>[4x]MVTALNYRVIDVDNHYYEPLDSFTRHLDKKFKRRGVQMLSDGKRTWAVIGDRVNHFIPNPTFDPIIVPGCLDLLFRGEIPDGVDPASLMKVERLADHPEYQNRDARIAVMDEQDIET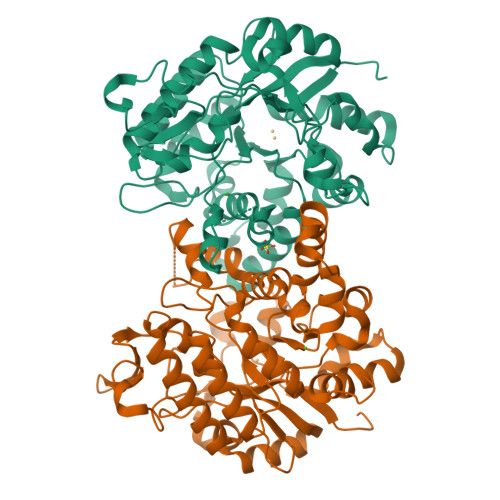AFMLPTFGCGVEEALKHDIEATMASVHAFNLWLDEDWGFDRPDHRIIAAPIVSLADPTRAVEEVDFVLARGAKLVLVRPAPVPGLVKPRSLGDRSHDPVWARLAEAGVPVGFHLSDSGYLHIAAAWGGKSTFEGFGAKDPLDQVLLDDRAIHDTMASMIVHGVFTRHPKLKAVSIENGSYFVHRLIKRLKKAANTQPQYFPEDPVEQLRNNVWIAPYYEDDLPELARVIGVDKILFGSDWPHGEGLASPVSFTAELKGFSESDIRKIMRDNALDLLGVQVGSAAAENLYFQSHHHHHHWSHPQFEK>[2x]MFNQFNPLV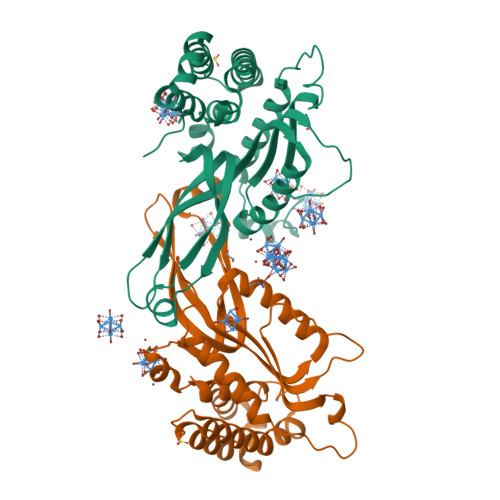YTHGGKLERKSKKDKTASKVFEEFGVMEAYNCWKEASLCIQQRDKDSVLKLVAALNTYKDAVEPIFDSRLNSAQEVLQPSILEEFFEYLFSRIDSIVGVNIPIRHPAKGYLSLSFNPHNIETLIQSPEYTVRAKDHDFIIGGSAKLTIQGHGGEGETTNIVVPAVAIECKRYLERNMLDECAGTAERLKRATPYCLYFVVAEYLKLDDGAPELTEIDEIYILRHQRNSERNKPGFKPNPIDGELIWDLYQEVMNHLGKIWWDPNSALQRGKVFNRP>HMDVDLAKSKVSAVSKQMNVPTEGAFKKFSAQVKFDPA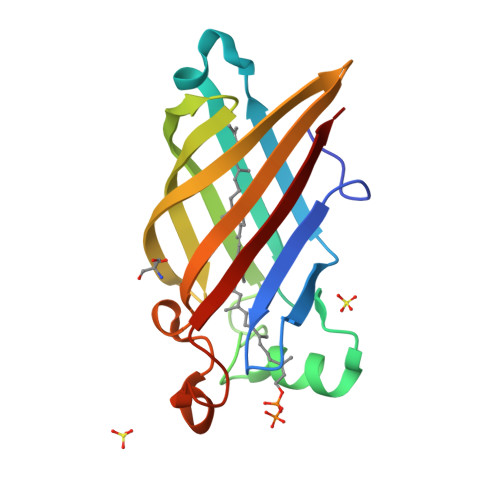KAAQGSAQMTIDVASFDLGDKMYNDQVAGKDWFDAKTYPQATFVSSAIAPAGGNKYNVTGKLTIKGKAETVTVPVTVAQNGATQTFDGVLPIKRSAFNVGTGEWKDTSIVADEVQIKFHLVAT[2x]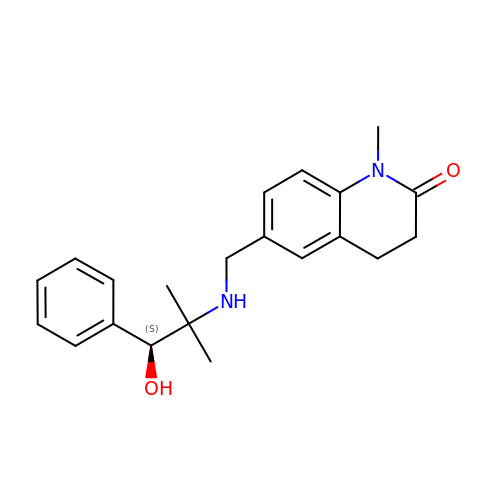6-({[(1S)-1-hydroxy-2-methyl-1-phenylpropan-2-yl]amino}methyl)-1-methyl-3,4-dihydroquinolin-2(1H)-one | C21 H26 N2 O2 | QITHCLWWRWXBDJ-FQEVSTJZSA-N We have studied this problem on the example of the mobile active site β1α1-loop (loop1) of the (βα)8-barrel enzyme HisF, which is the cyclase subunit of imidazole glycerol phosphate synthase. Prokaryotic ImGPS enzymes (including the ImGPS from T. maritima) form heterodimeric bienzyme complexes that consist of the cyclase HisF and the glutaminase HisH subunit, which supplies ammonia by glutamine hydrolysis. The active site of HisF is located at the C-terminal face of the central β-barrel, where two conserved aspartate residues, D11 and D130, catalyze the cyclase reaction. Based on the conformation of the loop that connects strand β1 with helix α1 (loop1), these structures can be separated into an open conformation, where loop1 is flipped toward the outer α-helical barrel ring, a detached conformation, where loop1 is not visible in the electron density and presumably flexible and a closed conformation, where loop1 closes over the active site.

To assess whether the mutations have an influence on the conformation of loop1 we determined the structures of the HisF-G20P and HisF-F23A variants by X-ray crystallography. In summary, our crystallography, proteolysis, NMR, and simulation data demonstrate that the HisF-G20P and HisF-F23A variants have opposing effects on the conformation of loop1. However, whereas loop1 primarily samples the open conformation in the HisF-G20P variant, the loop1 population shifts toward the highly flexible detached conformation in the HisF-F23A variant. Whereas the G20P and F23A substitutions decrease the kcat of wt-HisF by several orders of magnitude, the F38A substitution has no effect on the steady-state catalytic parameters. Instead, the G20P and F23A substitutions likely influence turnover via alterations in the closed conformation of loop1. In contrast, in the case of loop1 variants HisF-F23A and HisF-G20P, kobs, increased linearly with increasing concentrations of PrFAR, which is indicative of a simple binding process without involvement of conformational changes. The HisF-G20P and HisF-F23A variants on the other hand interact with the substrate via a one step binding mechanism as loop1 is, in those cases, unable to close properly over the substrate.

> LAKRIIACLDVKDGRVVKPTNFENLRDSGDPVELGKFYSEIGIDELVFLDITASVEKRKTMLELVEKVAEQIDIPFTVGGGIHDFETASELILRGADKVSINTAAVENPSLITQIAQTFGSQAVVVAIDAKRVDGEFMVFTYSGKKNTGILLRDWVVEVEKRGAGEILLTSIDRDGTKSGYDTEMIRFVRPLTTLPIIASGGAGKMEHFLEAFLAGADAALAASVFHFREIDVRELKEYLKKHGVNVRLEL> HHTFEYGDGI;> HHHHHHSSGLVPRGSHMAIYADNSYSIGNTPLVR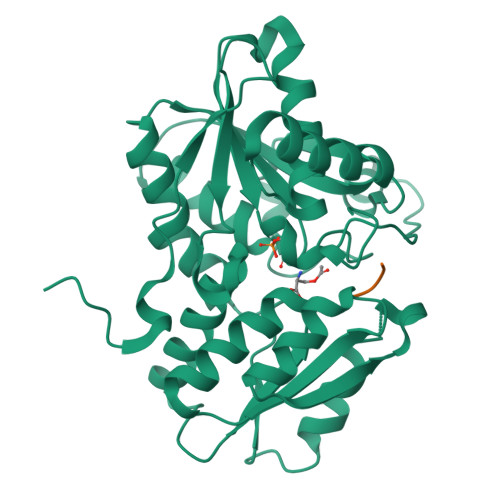LKHFGHNGNVVVKIEGRNPSYSVKCRIGANMVWQAEKDGTLTKGKEIVDATSGNTGIALAYVAAARGYKITLTMPETMSLERKRLLCGLGVNLVLTEGAKGMKGAIAKAEEIVASDPSRYVMLKQFENPANPQIHRETTGPEIWKDTDGKVDVVVAGVGTGGSITGISRAIKLDFGKQITSVAVEPVESPVISQTLAGEEVKPGPHKIQGIGAGFIPKNLDLSIIDRVETVDSDTALATARRLMAEEGILAGISSGAAVAAADRLAKLPEFADKLIVVILPSASERYLSTALFEGIEG>[2x]GHMKKQLIEFVRWSPERAQHYRNKGYWIDQPLTRILTVGVQSHPHSLAIICGERQLSYIELDRLSTNLATRLAEKGLGKGDTALVQLPNVAEFYIVFFALLKAGVVVLNALYSHRQYELNAFIKQIQPKLLIGSRQHEVFSNNQFIDSLHDVNLSPEIILMLNHQATDFGLLDWIETPAET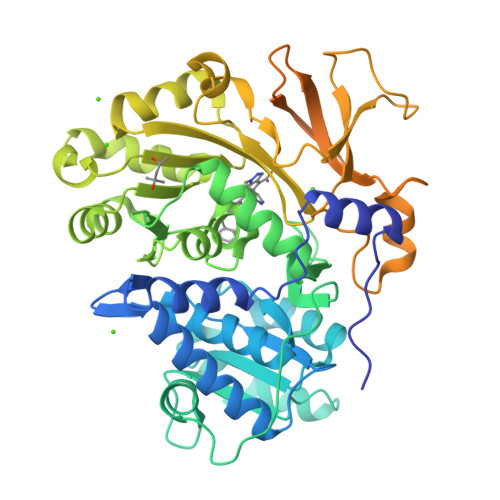FVDFSSTPADEVAFFQLSGGSTGTPKLIPRTHNDYDYSVRASAEICGLNSNTRLLCALPAPHNFMLSSPGALGVLHAGGCVVMAPNPEPLNCFSIIQRHQVNMASLVPSAVIMWLEKAAQYKDQIQSLKLLQVGGASFPESLARQVPEVLNCKLQQVFGMAEGLVNYTRLDDSDEQIFTTQGRPISSDDEIKIVDEQYREVPEGEIGMLATRGPYTFCGYYQSPEHNSQVFDEDNYYYSGDLVQRTPDGNLRVVGRIKDQINRGGEKIASEEIEKLILLHPEVMHAALVAIVDEQFGEKSCAFIVSRNPELKAVVLRRHLMELGIAQYKLPDQIKLIESLPLTAVGKVDKKQLRSILNTSTTS Phloxine B | C20 H3 Br4 Cl4 O5 | 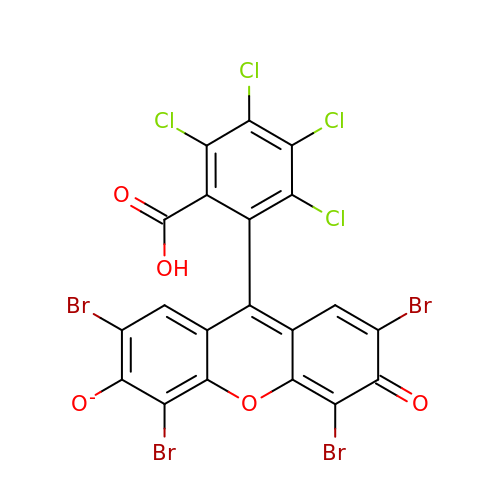RIVZUHBWXRGVOG-UHFFFAOYSA-M B. burgdorferi BBK32 is a surface-exposed lipoprotein with multiple roles in vertebrate host interactions. While the interaction of BBK32 with fibronectin and glycosaminoglycans is formed by non-overlapping binding sites in the intrinsically disordered N-terminal region of BBK32 (BBK32-N), the globular C-terminal region of BBK32 (BBK32-C) is now known to bind specifically to the initiating protease of the classical complement pathway, C1r. Previously we have shown that the C-terminal globular domain of B. burgdorferi BBK32 (termed BBK32-C) blocks classical pathway activation by binding with high-affinity to the initiating serine protease C1r, and preventing both its autocatalytic and C1s cleavage activities within the C1 complex. In fact, there are relatively few examples of pathogenic strategies which specifically target the classical pathway and BBK32 is the only known inhibitor which directly blocks the initiator protease C1r.

Preliminary limited proteolysis experiments suggested that flexible residues were present at the N- and C-termini in BBK32-C. A number of constructs were designed to truncate BBK32, ultimately yielding a C-terminal truncation mutant lacking six residues (i.e. BBK32(206–348)) which produced protein crystals. Importantly, the BBK32(206–348) construct retained full C1-binding, C1r-binding and complement inhibitory activities. BBK32(206–348) crystals grew in space group P65 with one molecule per asymmetric unit and diffracted to 1.7 Å resolution. BBK32(206–348) consists of five α-helices and adopts a helical bundle fold. Starting from the N-terminus, helix α1 (residues Ser-211 to Met-245) interacts with helices α3 (Lys- 256 to Ala-286), α4 (Ile-293 to Lys-317), and α5 (Leu-323 to Ile-347) to form an anti-parallel four-helix bundle. Helix α2 (Asn-251 to Ala-261) does not participate in the core bundle motif but rather forms hydrophobic interactions with helix α1 and sits at an angle of ~120° relative to helix 3. The protein surface is characterized by several contiguous positively charged regions with a larger negatively charged surface being formed where the C-terminal and N-terminal helices meet. Overall the structure of BBK32-C is best characterized by a positively charged anti-parallel four helix bundle where a fifth helix, helix α2, protrudes away from the helical core. In the BBK32-C structure E308 is a surface exposed residue located midway through α4, while Q319 and E324 are in the short loop connecting α4 and α5. Q319 and E324 are also surface exposed and together present a contiguous surface region.

> GSTGSSNRYQSYLEGVKYNVDSAIQTITKIYNTYTLFSTKLTQMYSTRLDNFAKAKAKEEAAKFTKEDLEKNFKTLLNYIQVSVKTAANFVYINDTHAKRKLENIEAEIKTLIAKIKEQSNLYEAYKAIVTSILLMRDSLKEVQGIID> TTEENSKSEALLDIPMLEQYLELVGPKLITDGLAVFEKMMPGYVSVLESNLTAQDKKGIVEEGHKIKGAAGSVGLRHLQQLGQQIQSPDLPAWED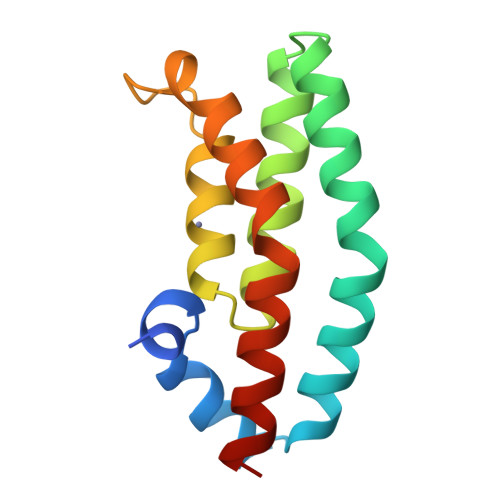NVGEWIEEMKEEWRHDVEVLKAWVAKATKK>MEHRAFKWPQPLAGNKPRIWYGGDYNPDQWPEEVWDEDVALMQQAGVNLVSVAIFSWAKLEPEEGVYDFDWLDRVIDKLGKAGIAVDLASGTASPPMWMTQAHPEILWVDYRGDVCQPGARQHWRATSPVFLDYALNLCRKMAEHYKDNPYVVSWHVSNEYGCHNRFDYSEDAERAFQKWCEKKYGTIDAVNDAWGTAFWAQRMNNFSEIIPPRFIGDGNFMNPGKLLDWKRFSSDALLDFYKAERDALLEIAPKPQTTNFMVSAGCTVLDYDKWGHDVDFVSNDHYFSPGEAHFDEMAYAACLTDGIARKNPWFLMSHSTSAVNWRPTNYRLEPGELVRDSLAHLAMGADAICYFQWRQSKAGAEKWHSAMVPHAGPDSQIFRDVCELGADLNKLADEGLLSTKLVKSKVAIVFDYESQWATEHTATPTQEVRHWTEPLDWFRALADNGLTADVVPVRGPWDEYEAVVLPSLAILSEQTTRRVREYVANGGKLFVTYYTGLVDDRDHVWLGGYPGSIRDVVGVRVEEFAPMGTDAPGTMDHLDLDNGTVAHDFADVITSVADTAHVVASFKADKWTGFDGAPAITVNDFGDGKAAYVGARLGREGLAKSLPALLEELGIETSAEDDRGEVLRVERADETGENHFVFLFNRTHDVAVVDVEGEPLVASLAQVNESEHTAAIQPNGVLVVKLAAALEHHHHHH[2x]

Aim: Bifidobacterium longum subsp. infantis uses a glycoside hydrolase (GH) family 42 β-galactosidase (BiBga42A) for hydrolyzing lacto-N-tetraose (LNT), which is the most abundant core structure of human milk oligosaccharides (HMOs). As such, BiBga42A represents one of the pivotal enzymes underpinning the symbiosis between bifidobacteria and breastfed infants. BiBga42A has a three-dimensional structure similar to other GH42 enzymes that have three domains consisting of a (β/α)8 barrel (domain A), an α/β fold (domain B), and an anti-parallel β-sandwich (domain C). Glu-160 and Glu-318 in BiBga42A were predicted to be the acid/base catalyst and the nucleophile, respectively, based on previous studies of GH42 enzymes and sequence alignment.

As a result, the lowest activity was detected for the E318S mutant. An LNT-complexed crystal was indeed obtained for the mutant, and the structure was determined at 2.2 Å resolution (E318S-LNT). The asymmetric unit of the E318S-LNT crystal contained two molecules (chains A and B) of BiBga42A, and they are virtually the same (Cα RMSD = 0.106 Å). The electron density map of LNT was clearly visible at the active site. The pyranose sugar ring of the Gal moiety in subsite -1 adopts a slightly distorted conformation toward OH5, and the C6 hydroxymethyl group takes a gg rotamer conformation. The carboxyl group of Glu-160 is suitably poised for proton donation to the leaving group as it is located 3.3 Å from the glycosidic bond oxygen of the LNB (Galβ1-3GlcNAc) unit in LNT. The C1 atom of the Gal moiety at subsite -1 in E318S-LNT has moved away from the side chain of Ser-318 with a distance of 6.2 Å. In addition, the C1 atom was located 4.3 Å from the nearest side chain oxygen atom (Oε1) of the superimposed Glu-318 of WT-GOL, and the configuration was not suitable for the in-line nucleophilic attack to the anomeric carbon. These observations might suggest that LNT was bound in a catalytically incompetent mode in the structure. The sugar ring of the GlcNAc in subsite +1 forms a stacking interaction with the side chain of Trp-326. The nitrogen atom of the N-acetyl group is recognized by a direct hydrogen bond with the carboxyl group of Glu-160 (the catalytic acid/base).> GSMLRLSAPGQLDDDLCLLGDVQVPVFLLRLGEASWALVEGGISRDAELVWADLCRWVADPSQVHYW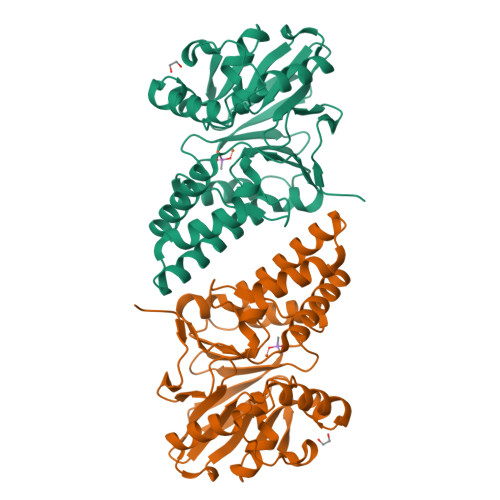LITHKHYDHCGLLPYLCPRLPNVQVLASERTCQAWKSESAVRVVERLNRQLLRAEQRLPEACAWDALPVRAVADGEWLELGPRHRLQVIEAHGHSDDHVVFYDVRRRRLFCGDALGEFDEAEGVWRPLVFDDMEAYLESLERLQRLPTLLQLIPGHGGLLRGRLAADGAESAYTECLRLCRRLLWRQSMGESLDELSEELHRAWGGQSVDFLPGELHLGSMRRMLEILSRQALPLD>[2x]QPVKRSIIAQDMFKTAFKGFKDGISAKCPKDTRLYSPDIQE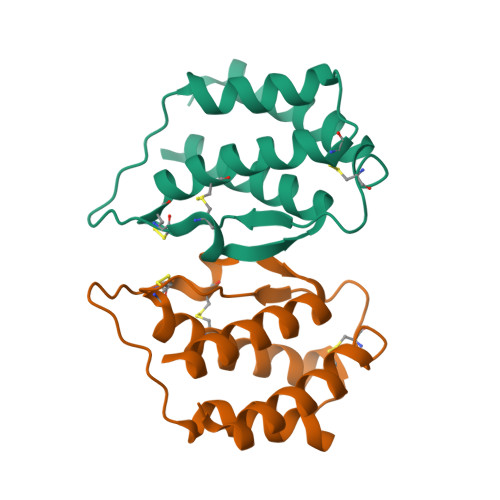DCLSSALKCTIAELKVLEVECNVTENDDFMMIYEGLNKEKWNTSSSSPRNCTCELYNQTHVKEFVENMERLVQLLYTRTQ>[4x]MVFTQAPAEIMGHLRIRSLLARQCLAEFLGVFVLMLLTQGAVAQAVTSGETKGNFFTMFLAGSLAVTIAIYVGGNVSGAHLNPAFSLAMCIVGRLPWVKLPIYILVQLLSAFCASGATYVLYHDALQNYTGGNLTVTGPKETASIFATYPAPYLSLNNGFLDQVLGTGMLIVGLLAILDRRNKGVPAGLEPVVVGMLILA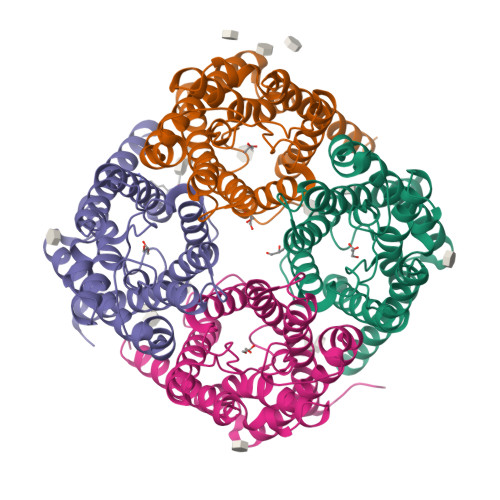LGLSMGANCGIPLNPARDLGPRLFTYVAGWGPEVFSAGNGWWWVPVVAPLVGATVGTATYQLLVALHHPEGPEPAQDLVSAQHKASELETPASAQMLECKL> CQDVVQDVPNVDVQMLELYDRMSFKDIDGGVWKQGWNIKYDPLKYNAHHKLKVFVVPHSHNDPGWIQTFEEYYQHDTKHILSNALRHLHDNPEMKFIWAEISYFARFYHDLGENKKLQMKSIVKNGQLEFVTGGWVMPDEANSHWRNVLLQLTEGQTWLKQFMNVTPTASWAIDPFGHSPTMPYILQKSGFKNMLIQRTHYSVKKELAQQRQLEFLWRQIWDNKGDTALFTHMMPFYSYDIPHTCGPDPKVCCQFDFKRMGSFGLSCPWKVPPRTISDQNVAARSDLLVDQWKKKAELYRTNVLLIPLGDDFRFKQNTEWDVQRVNYERLFEHINSQAHFNVQAQFGTLQEYFDAVHQAERAGQAEFPTLSGDFFTYADRSDNYWSGYYTSRPYHKRMDRVLMHYVRAAEMLSAWHSWDGMARIEERLEQARRELSLFQHHDGITGTAKTHVVVDYEQRMQEALKACQMVMQQSVYRLLTKPSIYSPDFSFSYFTLDDSRWPGSGVEDSRTTIILGEDILPSKHVVMHNTLPHWREQLVDFYVSSPFVSVTDLANNPVEAQVSPVWSWHHDTLTKTIHPQGSTTKYRIIFKARVPPMGLATYVLTISDSKPEHTSYASNLLLRKNPTSLPLGQYPEDVKFGDPREISLRVGNGPTLAFSEQGLLKSIQLTQDSPHVPVHFKFLKYGVRSHGDRSGAYLFLPNGPASPVELGQPVVLVTKGKLESSVSVGLPSVVHQTIMRGGAPEIRNLVDIGSLDNTEIVMRLETHIDSGDIFYTDLNGLQFIKRRRLDKLPLQANYYPIPSGMFIEDANTRLTLLTGQPLGGSSLASGELEIMQDRRLASDDERGLGQGVLDNKPVLHIYRLVLEKVNNCVRPS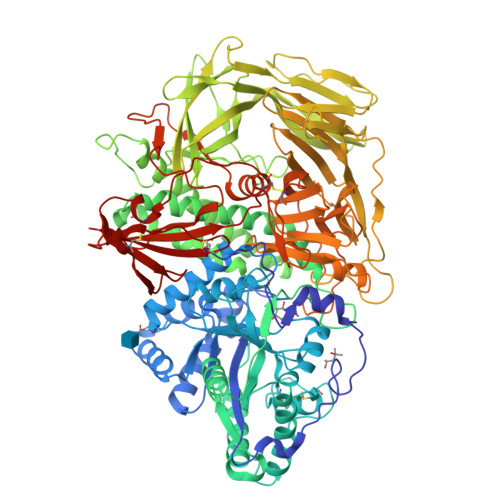KLHPAGYLTSAAHKASQSLLDPLDKFIFAENEWIGAQGQFGGDHPSAREDLDVSVMRRLTKSSAKTQRVGYVLHRTNLMQCGTPEEHTQKLDVCHLLPNVARCERTTLTFLQNLEHLDGMVAPEVCPMETAAYVSSHSS> GUUAUGUGUGCCCGGCAUGGGUGCAGUCUAUAGGGUGAGAGUCCCGAACUGUGAAGGCAGAAGUAACAGUUAGCCUAACGCAAGGGUGUCCGUGGCGACAUGGAAUCUGAAGGAAGCGGACGGCAAACCUUCGGUCUGAGGAACACGAACUUCAUAUGAGGCUAGGUAUCAAUGGAUGAGUUUGCAUAACAAAACAAAGUCCUUUCUGCCAAAG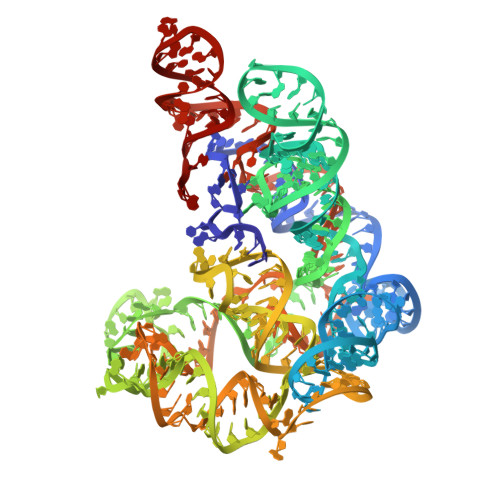UUGGUACAGAGUAAAUGAAGCAGAUUGAUGAAGGGAAAGACUGCAUUCUUACCCGGGGAGGUCUGGAAACAGAAGUCAGC> TGDVCKEKICSCNEIEGDLHVDCEKKGFTSLQRFTAPTSQFYHLFLHGNSLTRLFPNEFANFYNAVSLHMENNGLHEIVPGAFLGLQLVKRLHINNNKIKSFRKQTFLGLDDLEYLQADFNLLRDIDPGAFQDLNKLEVLILNDNLISTLPANVFQYVPITHLDLRGNRLKTL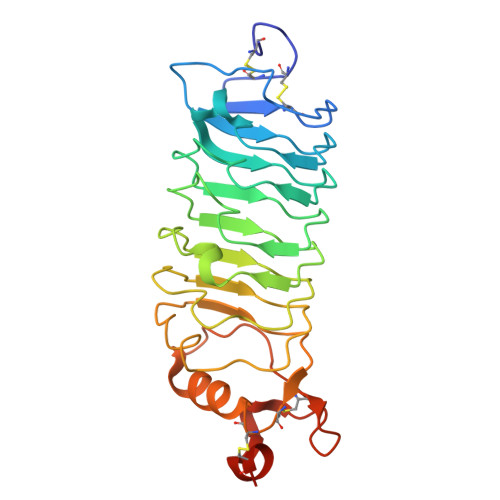PYEEVLEQIPGIAEILLEDNPWDCTCDLLSLKEWLENIPKNALIGRVVCEAPTRLQGKDLNETTEQDLCPLKSRLVPR> MSLDGTVLLIDYFEYEREKTKIIFDNIGEYDFIEVENLKKFYSIFKDLDSITLIIMDIAFPVEKEGLEVLSAIRNNSRTANTPVIIATKSDNPGYRHAALKFKVSDYILKPYPTKRLENSVRS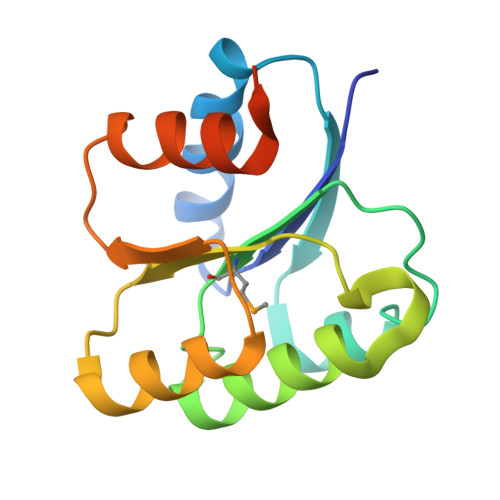VLKICQRFREGHHHHHH> QELPQMTQQLNSDDMQEQLSATVKFRQILSREHRPPIDVVIQAGVVPRLVEFMRENQPEMLQLEAAWALTNIASGTSAQTKVVVDADAVPLFIQLLYTGSVEVKEQAIWALGNVAGDSTDYRDYVLQCNAMEPILGLFNSNKPSLIRTATWTLSNLCRGKKPQPDWSVVSQALPTLAKLIYSMD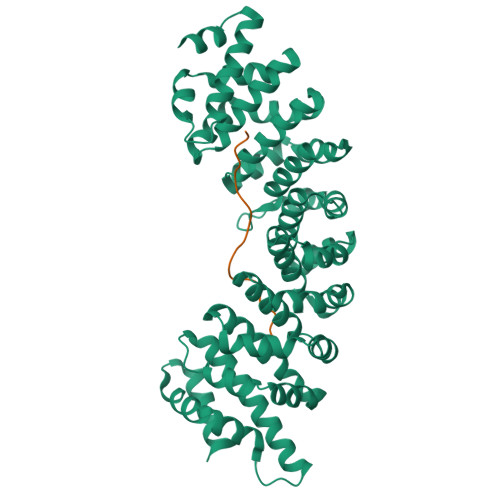TETLVDACWAISYLSDGPQEAIQAVIDVRIPKRLVELLSHESTLVQTPALRAVGNIVTGNDLQTQVVINAGVLPALRLLLSSPKENIKKEACWTISNITAGNTEQIQAVIDANLIPPLVKLLEVAEDKTKKEACWAISNASSGGLQRPDIIRYLVSQGCIKPLCDLLEIADNRIIEVTLDALENILKMGEADKEARGLNINENADFIEKAGGMEKIFNCQQNENDKIYEKAYKIIETYFG;> AVKRPAATKKAGQAKKKKL> MVIDSKQDLPQYTKDSGSESDSDSSNNFIVESPSIPSSKSATVVLNSEEYEDDEGDDLNGLDAELIDNITYEGDEDETMFVGLKEKQKLHLSGVFRLQVVKGGIVYNNVHYNASREILTFWHPLSQSIPTIDFSHFAGWQDTFFMPRNNRFKIRDEEFKSFPCVLRVFNSNHTGLLEAGHLYRDVNYLWKPKEPYFPLNERTTYHLLHESDRIQSLSVPGYWSTPLEKLYLSHKNAAYDTRIMVIGGKNSGKSTFLRLLLEKFTQDIRDSTTSQEELVYLDLDPGQPEYSLPDSISLNKILSSPISLGQHLCQGSNFQTLLQFYAGSSSPQDEPTSYLNCADKLIDHLEEQAFFGTSLLNLPGWIKGFGMQILNHIIRKYKPTHLLFLETANSKRHLDELTIPQSFSTSLRDAYAPEVVRVPAHS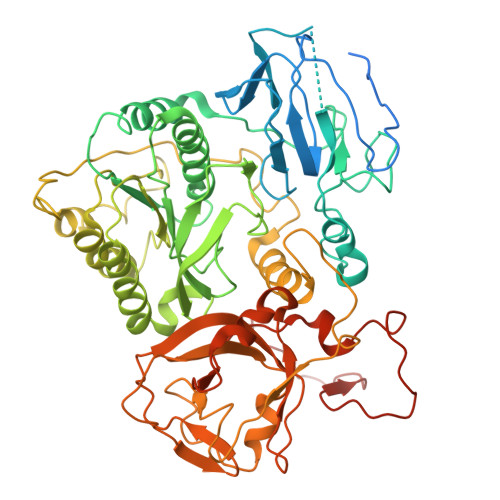LNHTLSSRFHASQLRTFKILALFHKITQFDYDFAPLLKSAPLQISYGKGKSGIKGIQFPMEFQDLNPQDIKSALEGTVIGIYTYSGEDSLEVKSLNTFPILQSCTSSSKNFITLGLIHSIDTSQQIMNIYVPPCHTQILDKQPEDAQWIIVRNKTETPFCDFLPSPRTITWDDNIQIPFATFERRKKLEHVWKVRKNVMRRGQFMKR>[8x]MGYFDHVGTVKFEGKSSTNPLAFKFYNPDEIILGKTMREHLRFGVAYWHSFTGNGSDPFGAGTALRGWNELSGMELAKARVEACFELLNILDVDYFCFHDRDIAPEGDTLQETNRNLDEIVALIKQHMHSSGKKLLWNTANMFTNPRFVHGAATTSNADVFAYAAAQVKKALDHGKELGAENYVFWGGREGYESLLNTDLGLELDNLAR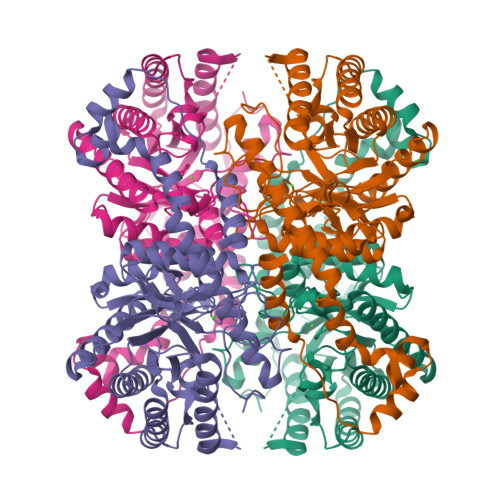FLQLAVDYAKEIGFDAQFLIEPKPKEPSKHQYDFDAATTLQFLQKYDLAKHFKLNLEANHATLAGHTFEHELRVARINGALGSIDANQGDLLLGWDTDEFPTDLYASTLAMYEILQNEGGIGRGGVNFDAKVRRTSFEPIDVVYAHINGMDAFARGLQVAAKLIEDRAFDNVIEERYASFTKGIGADIVSGKANFHTLEAYALQNNPITNKSGRVELLRSILNQYIINV NAMPT functions as a homo-dimeric enzyme that catalyzes the rate limiting step in the primary salvage pathway for NAD synthesis, the transfer of a phosphoribosyl residue from 5-phosphoribosyl-1-pyrophosphate (PRPP) to nicotinamide (NAM) to produce nicotinamide mononucleotide (NMN). Crystal structures of NAMPT in numerous ligand-bound forms have been reported. These structures consistently display a NAMPT homo-dimer with two essentially identical active sites at the dimer interface. Typical NAMPT inhibitors were found to occupy the portion of active site responsible for NAM binding and a tunnel-shaped cavity extending from the NAM binding site. Furthermore, we determine the crystal structures of six NAMPT mutants in the apo form and in complex with various inhibitors and present a definitive model to explain the differential effects of the mutations on various structural classes of NAMPT inhibitors.

A previously published in silico model predicted that H191R would protrude its side chain into the tunnel and sterically block inhibitors like APO866 from binding. When tested across a panel of structurally diverse inhibitors, H191R reduced potency across the compound families, but remained more sensitive to APO866 and GMX1778 than series A inhibitors. The R191 side chain indeed occupied part of the volume inside the tunnel region, but did not completely block the tunnel passage, thus imposing a more stringent limit on the size of linker moieties in the inhibitor molecules. The bi-aryl sulfone group of series A compounds exceeded the available space, whereas the more flexible and narrower linker of APO866 can fit through the altered tunnel.

>MNPAAEAEFNILLATDSYKVTHYKQYPPNTSKVYSYFECREKKTENSKLRKVKYEETVFYGLQYILNKYLKGKVVTKEKIQEAKDVYKEHFQDDVFNEKGWNYILEKYDGHLPIEIKAVPEGFVIPRGNVLFTVENTDPECYWLTNWIETILVQSWYPITVATNSREQKKILAKYLLETSGNLDGLEYKLRDFGYRGVSSQETAGIGASAHLVNFKGTDTVAGLALIKKYYGTKDPVPGYSVPAAEHSTITAWGKDHEKDAFEHIVTQFSSVPVSVVSDSYDIYNACEKIWGEDLRHLIVSRSTQAPLIIRPDSGNPLDTVLKVLEILGKKFPVTENSKGYKLLPPYLRVIQGDGVDINTLQEIVEGMKQKMWSIENIAFGSGGGLLQKLTRDLLNCSFKCSYVVTNGLGINVFKDPVADPNKRSKKGRLSLHRTPAGNFVTLEEGKGDLEEYGQDLLHTVFKNGKVTKSYSFDEIRKNAQLNIELEAAHHLEHHHHHHHH[2x]>MEPELNKERPSLQIKLKIEDFELHKMLGKGSFGKVFLAEFKKTNQFFAIKALKKDVVLMDDDVECTMVEKRVLSLAWEHPFLTHMFCTFQTKENLFFVMEYLNGGDLMYHIQSCHKFDLSRATFYAAEIILGLQFLHSKGIVYRDLKLDNILLDKDGHIKIADFGMCKENMLGDAKTNEFCGTPDYIAPEILLGQKYNHSVDWWSFGVLLYEMLIGQSPFHGQDEEELFHSIRMDNPFYPRWLEKEAKDLLVKLFVREPEKRLGVRGDIRQHPLFREINWEELERKEIDPPFRPKVKSPFDCSNFDKEFLNEKPRLSFADRALINSMDQNMFRNFSFMNPGMER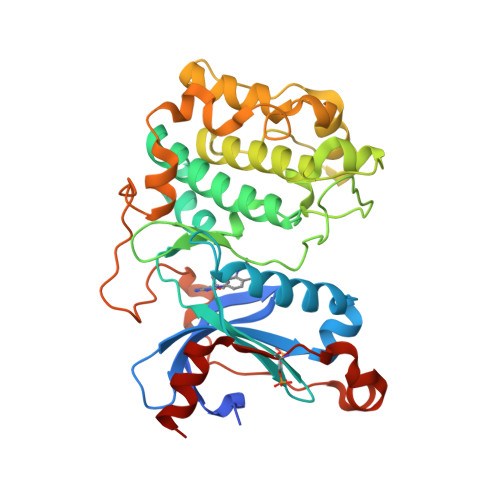LISHHHHHH[2x]>[2x]MPLLVEGRRVRLPQSAGDLVRAHPPLEERAR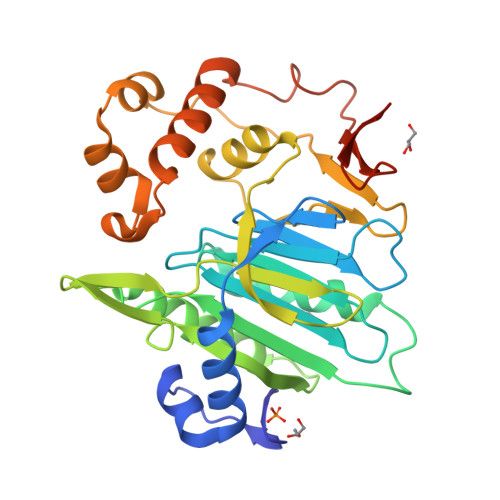LLRGQSVQQVGPQGLLYVQQRELAVTSPKDGSISILGSDDATTCHIVVLRHTGNGATCLTHCDGTDTKAEVPLIMNSIKSFSDHAQCGRLEVHLVGGFSDDRQLSQKLTHQLLSEFDRQEDDIHLVTLCVTELNDREENENHFPVIYGIAVNIKTAEIYRASFQDRGPEEQLRAARTLAGGPMISIYDAETEQLRIGPYSWTPFPHVDFWLHQDDKQILENLSTSPLAEPPHFVEHIRSTLMFLKKHPSPAHTLFSGNKALLYKKNEDGLWEKISSPGSLEHHHHHH>GSLSDQLSKQTLLISQLQVGKNRFSFKFEGRVVYKSSTFQNQQDSKYFFITAQDANNQEINLSFWQKVDQSYQTLKVGQYYYFIGGEVKQFKNNLELKFKFGDYQIIPKETLGGSGGSTLLISEVLKTSKQYLSVLAQVVDIQSSDKNIRLKICDNSCNQELKVVIFPDLCYEWRDKFSINKWYYFNEFVRQIY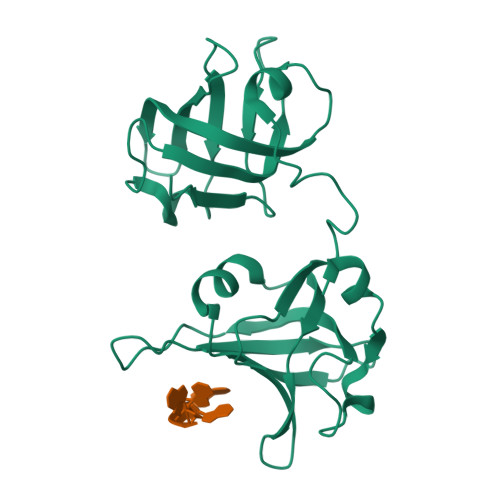NDEVQLKNNIHSSIKESDD[4x]> GTGDGSELPKEMEEYFEMLQREIDKAYEIAKKARAQGKDPSLDVEIPQATDMAGRVESLVGPPGVAKRIRELVKEYGKEIAALKIVDEIIEGKFGDLGSREKYAEQAVRTALAILTEGIVSAPIEGIANVKIKRNTWADNSEYLALYYAGPIRSSGGTAQALSVLVGDYVRRKLGLDRFKPSEKHIERMVEEVDLYHRAVTRLQYHPSPEEVRLAMRNIPIEITGEATDDVEVSHRDVPGVETNQLRGGAILVLAEGVLQKAKKLVKYIDKMGIEGWEWLKEFVEAKEKGEPKEEGKEESLAESTLEETKVEVDMGFYYSLYQKFKEEIAPSDKYAKEVIGGRPLFSDPSKPGGFRLRYGRSRASGFATWGINPATMILVDEFLAIGTQLKTERPGKGAVVTPVTTIEGPIVKLKDGSVLRVDDYNLALKVREDVEEILYLGDAVIAFGDFVENNQTLLPANYCEEWWILEFVKALKEIYEVHLEPFTENEEESIEEASDYLEIDPEFLKEMLRDPLRVKPPVELAIHFSEVLGIPLHPYYTLYWNSVEPKDVEKLWRLLKNYAEIEWSNFRGIKFAKKIVISQEKLGDSKRTLELLGLPHTVRDGNVIVDYPWAAALLTPLGNLNWEFMAKPLYATIDIINENNEIKLRDRGISWIGARMGRPEKAKERKMKPPVQVLFPIGLAGGSSRDIKKAAEEGKVAEVEIAFFKCPKCGHVGPEHLCPNCGTRKELLWVCPRCNAEYPESQAEGYNYTCPKCNVKLRPYAKRKIRPSELLNRAMENVKVYGVDKLKGVMGMTSGWKMPEPLEKGLLRAKNDVYVFKDGTIRFDATDAPITHFRPREIGVSVEKLRELGYTHDFEGKPLVSEDQIVELKPQDIILSKEAGRYLLKVAKFVDDLLEKFYGLPRFYNAEKMEDLIGHLVIGLAPHTSAGIVGRIIGFVDALVGYAHPYFHAAKRRNCDGDEDAVMLLLDALLNFSRYYLPEKRGGKMDAPLVITTRLDPREVDSEVHNMDIVRYYPLEFYEATYELKSPKELVGVIERVEDRLGKPEMYYGLKFTHDTDDIAL

PolD exists in all Archaea, except Crenarchaea, and is a replicative polymerase responsible for initiating DNA synthesis at both leading and lagging strands5678. It is composed of a large catalytic subunit (DP2) and a smaller subunit with 3′–5′ proofreading exonuclease activity (DP1)5. To help resolve the uncertainty concerning the evolutionary origins of D-family DNAP, we determined the crystal structures of two large fragments of both DP1 and DP2 subunits of the Pyrococcus abyssi PolD. While the interaction between the two subunits is essential for the full activity of PolD71413, both DP1 and DP2 constructs described here are capable of digesting mispaired 3′–5′ nucleotides and of extending a DNA primer in a templated manner, respectively. Both DP1 and DP2 crystal structures were determined individually by experimental phasing and refined at final resolutions of 2.5 and 2.2 Å, respectively.

The DP2 construct covers amino acids 1–1,050 from DP2 DNAP subunit, leaving out a C-terminal domain (CTD; 1,051–1,270) dedicated to interaction with DP1 (refs 13, 14). The DP2 structure reveals an extended molecule with overall dimensions of 55 × 60 × 110 Å3 and four domains: the N-terminal domain (NTD; residues 1–285), the central domain (residues 308–667), the catalytic domain (residues 668–996) and a fragment of the CTD (residues 997–1,039). The most prominent feature of the DP2 architecture is the extensive interaction between the NTD and catalytic domain, which results in a wide interfacial crevice that hosts the DNAP active site, formed by two double-psi β-barrels (DPBBs). Unexpectedly, PolD DP2 and ‘two-barrel' RNA polymerases (RNAPs) share a conserved architecture in their active sites. The peptide chain connecting the fifth (β31) and the sixth (β32) β-strands of the barrel forms a right-handed α-helix followed by a 10-residue-long loop, which constitutes the most conserved sequence motif of DP2. This motif comprises two invariant aspartic residues (D961 and D963), which were previously shown to be catalytically critical for PolD DNAP activity. The DPBB is preceded by a helical region composed of three α-helices (α24, α26–27) and a tandem repeat of two zinc modules, named Zn-I and Zn-II. In both cases, Zn2+ are tetrahedrally coordinated by two pairs of cysteines located in turns, but apart from that the two zinc-binding modules bear no structural relationship to each other. In particular, the peptide chains connecting the NTD to the central domain (residues 286–307), strands β7 to β8 (residues 358–364), strands β8 to β9 (residues 376–392) and strand β18 to the catalytic domain (residues 654–668) were not visible in the electron density. The 50 residues of the CTD present in our construct are partly disordered, except for two helices α32 and α33 (residues 1,011–1,039), which bind next to the interface between the central and catalytic domains through interactions with the DPPB-1 and helix α32.> ITGTSTVGVGRGVLGDQKNINTTYSTYYYLQDNTRGNGIFTYDAKYRTTLPGSLWADADNQFFASYDAPAVDAHYYAGVTYDYYKNVHNRLSYDGNNAAIRSSVHYSQGYNNAFWNGSQMVYGDGDGQTFIPLSGGIDVVAHELTHAVTDYTAGLIYQNESGAINEAISDIFGTLVEFYANKNPDWEIGEDVYTPGISGDSLRSMS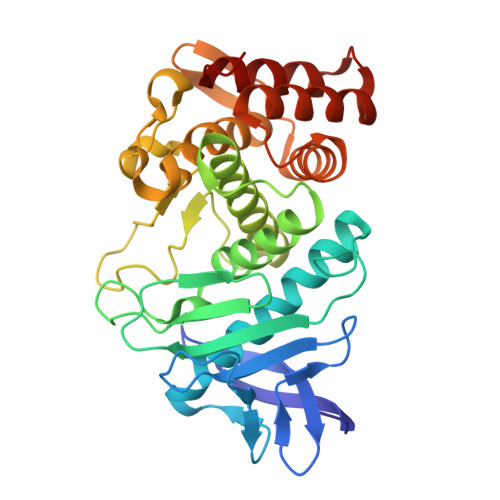DPAKYGDPDHYSKRYTGTQDNGGVHINSGIINKAAYLISQGGTHYGVSVVGIGRDKLGKIFYRALTQYLTPTSNFSQLRAAAVQSATDLYGSTSQEVASVKQAFDAVGVK Chemoeffectors are sensed by chemoreceptors that in turn stimulate chemosensory pathways that modulate the activity of the flagellar motor. A canonical chemoreceptor is composed of an extracytosolic ligand-binding domain (LBD) and a cytosolic region that contains the signaling domain that interacts with other signaling proteins. The dCache domain is the predominant extracellular LBD in bacterial signal transduction systems, and it is present in about 15% of all chemoreceptors. To identify the molecular determinants for acetylcholine recognition, we report high-resolution structures of PctD-LBD (with bound acetylcholine and choline) and PacA-LBD (with bound betaine).

We also identified the PacA (ECA_RS10935) chemoreceptor of the phytopathogen Pectobacterium atrosepticum, which binds choline and betaine but fails to recognize acetylcholine. Betaine bound most tightly (KD = 7.5 μM), followed by l-carnitine and choline with KD values of 20 μM and 113 μM, respectively. Importantly, titration with 5 mM acetylcholine did not produce any change in heat, indicating an absence of binding. We crystalized the PacA-LBD and solved its 3D structure in complex with betaine to a resolution of 1.9 Å. The overall structure is highly similar to that of PctD-LBD, with a root mean square deviation of 1.6 Å for the Cα atoms in a structural alignment. A well-defined electron density was observed for betaine bound to PacA-LBD. The orientation of betaine corresponded to that of acetylcholine in PctD-LBD, which was the opposite of the orientation of choline. The coordination of the quaternary amine moiety in PacA-LBD is very similar to that of PctD-LBD and primarily involves a number of aromatic amino acids. However, the amino acids that coordinate the acetylcholine tail in PctD-LBD (Ala168, Met169, Asp171, and Ser172) are not conserved in PacA-LBD. However, comparison of the three-dimensional structures of ligand-bound PctD-LBD and PacA-LBD identified the amino acids uniquely involved in acetylcholine recognition.

>[4x]MGSSHHHHHHSSGLVPRGSHSWQSSSEQKSLAERYLQQIAQSEALRIQQELNYARDVAHNLGQGLAALPSAGIKDRAVVDKMMEYALRDNPEYLSISVIFEENVFDGRDAEFADQPGQAPKGRYAWFVDRDQAGNYAMHPLLSYLTPGQGDYYLLPQKSQKDTLIEPYTYAYNGVPTLLTSVAAPIVSQGKLWGVVTSDISLASLQQKINQIKPWEGGGYAMLLSSAGKVISYPDKSQTSKAWQGPTDNFTSSVVQHDDAILGEQALVTWQPVTIGNSTEKWYLGIVVPVSQVMAASERQL> MVNISDFFGKNKKSVRSSTSRPTRQVGSSKPEVIDLDTESDQESTNKTPKKMPVSNVIDVSETPEGEKKLPLPAKRKASSPTVKPASSKKTKPSSKSSDSASNITAQDVLDKIPSLDLSNVHVKENAKFDFKSANSNADPDEIVSEIGSFPEGKPNCLLGLTIVFTGVLPTLERGASEALAKRYGARVTKSISSKTSVVVLGDEAGPKKLEKIKQLKIKAIDEEGFKQLIAGMPAEGGDGEAAEKARRKLEEQHNIATKEAELLVKKEEERSKKLAATRVSGGHLERDNVREEDKLWTVKYAPTNLQQVCGNKGSVMKLKNWLANWENSKKNSFKHAGKDGSGVFRAAMLYGPPGIGKTTAAHLVAQELGYDILEQNASDVRSKTLLNAGVKNALDNMSVVGYFKHNEEAQNLNGKHFVIIMDEVDGMSGGDRGGVGQLAQFCRKTSTPLILICNERNLPKMRPFDRVCLDIQFRRPDANSIKSRLMTIAIREKFKLDPNVIDRLIQTTRGDIRQVINLLSTISTTTKTINHENINEISKAWEKNIALKPFDIAHKMLDGQIYSDIGSRNFTLNDKIALYFDDFDFTPLMIQENYLSTRPSVLKPGQSHLEAVAEAANCISLGDIVEKKIRSSEQLWSLLPLHAVLSSVYPASKVAGHMAGRINFTAWLGQNSKSAKYYRLLQEIHYHTRLGTSTDKIGLRLDYLPTFRKRLLDPFLKQGADAISSVIEVMDDYYLTKEDWDSIMEFFVGPDVTTAIIKKIPATVKSGFTRKYNSMTHPVAIYRTGSTIGGGGVGTSTSTPDFEDVVDADDNPVPADDEETQDSSTDLKKDKLIKQKAKPTKRKTATSKPGGSKKRKTKA;> MSKTLSLQLPWVEKYRPQVLSDIVGNKETIDRLQQIAKDGNMPHMIISGMPGIGKTTSVHCLAHELLGRSYADGVLELNASDDRGIDVVRNQIKHFAQKKLHLPPGKHKIVILDEADSMTAGAQQALRRTMELYSNSTRFAFACNQSNKIIEPLQSRCAILRYSKLSDEDVLKRLLQIIKLEDVKYTNDGLEAIIFTAEGDMRQAINNLQSTVAGHGLVNADNVFKIVDSPHPLIVKKMLLASNLEDSIQILRTDLWKKGYSSIDIVTTSFRVTKNLAQVKESVRLEMIKEIGLTHMRILEGVGT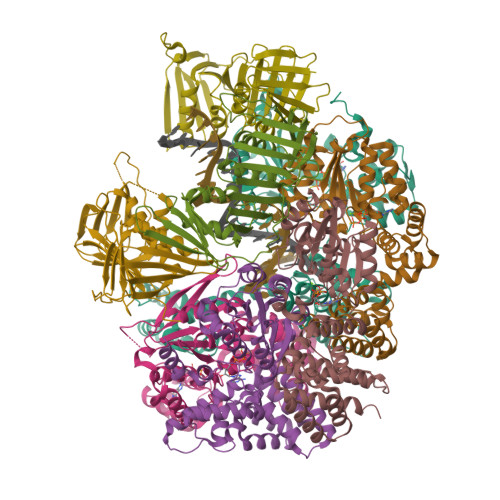YLQLASMLAKIHKLNNKA;> MSTSTEKRSKENLPWVEKYRPETLDEVYGQNEVITTVRKFVDEGKLPHLLFYGPPGTGKTSTIVALAREIYGKNYSNMVLELNASDDRGIDVVRNQIKDFASTRQIFSKGFKLIILDEADAMTNAAQNALRRVIERYTKNTRFCVLANYAHKLTPALLSRCTRFRFQPLPQEAIERRIANVLVHEKLKLSPNAEKALIELSNGDMRRVLNVLQSCKATLDNPDEDEISDDVIYECCGAPRPSDLKAVLKSILEDDWGTAHYTLNKVRSAKGLALIDLIEGIVKILEDYELQNEETRVHLLTKLADIEYSISKGGNDQIQGSAVIGAIKASFENETVKANV;> MFEGFGPNKKRKISKLAAEQSLAQQPWVEKYRPKNLDEVTAQDHAVTVLKKTLKSANLPHMLFYGPPGTGKTSTILALTKELYGPDLMKSRILELNASDERGISIVREKVKNFARLTVSKPSKHDLENYPCPPYKIIILDEADSMTADAQSALRRTMETYSGVTRFCLICNYVTRIIDPLASRCSKFRFKALDASNAIDRLRFISEQENVKCDDGVLERILDISAGDLRRGITLLQSASKGAQYLGDGKNITSTQVEELAGVVPHDILIEIVEKVKSGDFDEIKKYVNTFMKSGWSAASVVNQLHEYYITNDNFDTNFKNQISWLLFTTDSRLNNGTNEHIQLLNLLVKISQL;> MSLWVDKYRPKSLNALSHNEELTNFLKSLSDQPRDLPHLLLYGPNGTGKKTRCMALLESIFGPGVYRLKIDVRQFVTASNRKLELNVVSSPYHLEITPSDMGNNDRIVIQELLKEVAQMEQVDFQDSKDGLAHRYKCVIINEANSLTKDAQAALRRTMEKYSKNIRLIMVCDSMSPIIAPIKSRCLLIRCPAPSDSEISTILSDVVTNERIQLETKDILKRIAQASNGNLRVSLLMLESMALNNELALKSSSPIIKPDWIIVIHKLTRKIVKERSVNSLIECRAVLYDLLAHCIPANIILKELTFSLLDVETLNTTNKSSIIEYSSVFDERLSLGNKAIFHLEGFIAKVMCCLD;>[3x]GPHMASMLEAKFEEASLFKRIIDGFKDCVQLVNFQCKEDGIIAQAVDDSRVLLVSLEIGVEAFQEYRCDHPVTLGMDLTSLSKILRCGNNTDTLTLIADNTPDSIILLFEDTKKDRIAEYSLKLMDIDADFLKIEELQYDSTLSLPSSEFSKIVRDLSQLSDSINIMITKETIKFVADGDIGSGSVIIKPFVDMEHPETSIKLEMDQPVDLTFGAKYLLDIIKGSSLSDRVGIRLSSEAPALFQFDLKSGFLQFFLAPKFNDEE1-DEOXY-D-XYLULOSE-5-PHOSPHATE | C5 H11 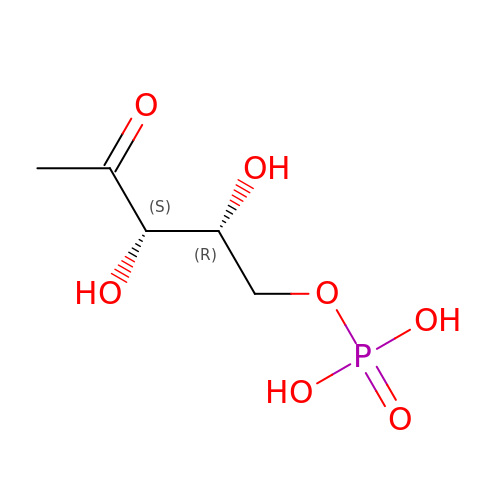O7 P | AJPADPZSRRUGHI-RFZPGFLSSA-N>[4x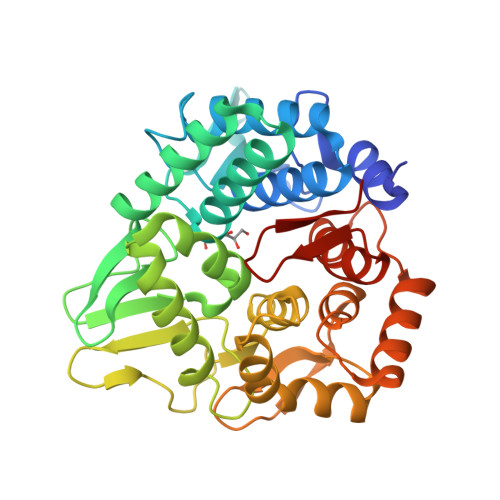]GSHMACTWPAWEHFKRAYISDGGRVIDPSDARKITTSEGQSYALFFALAADDRPMFDNVLEWTKDNLAQGDPGEHLPAWLWGKKDENNWTVLDSNSASDADIWIAWSLLEAGRLWKEARYTTLGNALLNRIAKEEVVTVPGLGPMLLPGKVGFAEETVWRLNPSYLPPQIARYLTRFGEPWTTLQETNHRLLLETAPKGFSPDWVRYEKSKGWQLAPDKTLISGYDAIRVYLWVGMMNDHDAQKASLLERLKPMAALTAKKGVVPEKVDVATAQPRGDGPVGFAAALLPFLQDRDAQAVQRQKVADHFPGDDAYFSYVLTLFGQGWDEHRFRFTPRGELQPDWGQACASSQ[(2~{Z},4~{E},6~{E},8~{E},10~{E},12~{E},14~{E})-17-[(4~{S},6~{R})-4-acetyloxy-2,2,6-trimethyl-6-oxidanyl-cyclohexylidene]-6,11,15-trimethyl-2-[(~{E})-2-[(1~{S},4~{S},6~{R})-2,2,6-trimethyl-4-oxidanyl-7-oxabicyclo[4.1.0]heptan-1-yl]ethenyl]heptadeca-2,4,6,8,10,12,14,16-octaenyl] octanoate | C50 H72 O7 | 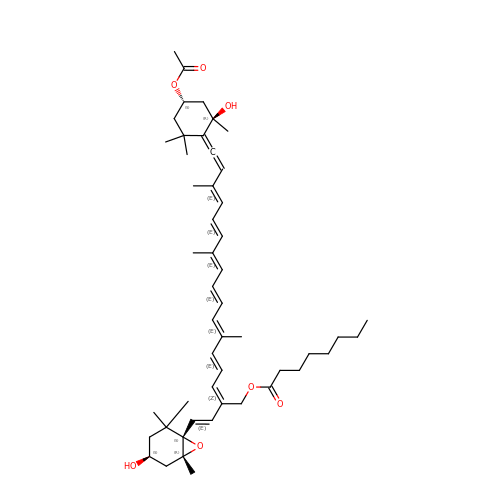JYJFYJLLQQTZBJ-AYSGSIDZSA-N>[4x]MKQTSLEVKEFALNLISQFEPENQPLGFWIFDTEGVEKAVERWKKNMPTVRPCFAVKCNPEPHLVKLLGELGCGFDCASLNEIKEVLDLGFNPEDITYSQTFKPYNQLIEASHLGINHTIVDSIDEVQKIAKYAPKMGIMIRIMENDTSAGHVFGEKFGLHDDEVEIVLKEIKDKGLNLDGVHFHVGSDSHNSEVFTKALTKARNTVTLAEQFGMKPYLIDIGGGFSQVAPFEEFAATIEKTIKELEFPERTRFIAEPGRYMASNAFHLVSSLHGKRVRIQNGKKQIEYTSGDGLHGSFGCCIWFEKQKSCECITQKVNENTKMYESIIYGPSCNGSDKVATQELPEMEPGKDWLLFPNMGAYTISMATNFNGFEERNHVIYTLPLKSTKIIQIP

Ornithine decarboxylase catalyzes the first and rate-limiting step of polyamine biosynthetic pathway. L-ornithine is decarboxylated by ODC enzyme in the presence of cofactor pyridoxal-5′-phosphate (PLP) to produce putrescine. The ODC enzyme is an obligate homodimer with two symmetry-related active sites located at the dimer interface. The ODC enzyme from E. histolytica belongs to fold type III group IV decarboxylase of a B6-dependent family, having eukaryotic ornithine decarboxylase characteristics.

Here, we report cloning, purification and crystal structure determination of C-terminal truncated Entamoeba histolytica ornithine decarboxylase (EhODCΔ15). The crystal diffracted to 2.8 Å resolution, possessing four molecules per asymmetric unit and the solvent content was calculated to be 46.69% with a Matthews coefficient of 2.2 Å3 Da−1. The four monomers in the asymmetric unit of crystal are arranged as two separate dimers (subunits A, B and subunits C, D) facing each other at the convex surfaces. Each monomer consists of β/α barrel and β-sheet domain which are arranged identical to previously known ODC structures. As expected, the crystal structure of EhODC contains two equivalent active site pockets at the dimer interface formed by residues that are contributed from both the subunits. In contrast, Cys'334 the conserved residue of EhODC that is expected to form a covalent bond with DFMO is slightly displaced from its position and has distinct orientation that is structurally unfavourable for covalent linkage with DFMO. In addition, the residue Asp'361 of TbODC is substituted by Asn'335 in EhODC, which is not expected to interact with DFMO. Tyr'323 is replaced with His'296 in EhODC and the loop containing His'296 residue is positioned away from the active site. In contrast, the cofactor PLP and substrate L-ornithine are accommodated in EhODC active site with polar interactions to facilitate the catalysis. These structural details indicate that amino acid substitutions in the active site of EhODC create a novel architecture which not only makes it resistant to DFMO but also lowers its catalytic efficiency by weakening substrate binding, as the reported Km values for L-ornithine for active but DFMO sensitive T. brucei and mouse ODC enzymes are 0.24 mM and 0.09 mM respectively, whereas for DFMO resistant EhODC it is 1.5 mM. Structure of EhODC at 2.8 Å revealed two salt bridges between Lys157-Asp238 at a distance 2.9 Å and Asp122-Arg277 at 3.2 Å.>[2x]HHHHHHMKDRFELVSKYQPQGDQPKAIEKLVKGIQEGKKHQTLLGATGTGKTFTVSNLIKEVNKPTLVIAHNKTLAGQLYSEFKEFFPNNAVEYFVSYYDYYQPEAYVPQTDTFIEKDASINDEIDKLRHSATSALFERRDVIIIASVSCIYGLGSPEEYREMVVSLRTEMEIERNELLRKLVDIQYARNDIDFQRGTFRVRGDVVEIFPASRDEHCVRVEFFGDEIERIREVDALTGEILGDRDHVAIFPASHFVTRAEK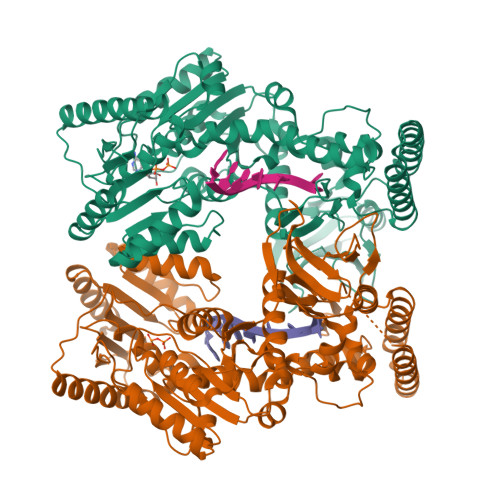MEKAIQNIEKELEEQLKVMHENGKLLEAQRLEQRTRYDLEMMREMGFCSGIENYSRHLTLRPPGSTPYTLLDYFPDDFMIVVDESHVTIPQVRGMFNGDQARKQVLVDHGFRLPSALDNRPLRFEEFEKHMHNIVYVSATPGPYEIEHTDEMVEQIIRPTGLLDPLIDVRPIEGQIDDLIGEIQARIERNERVLVTTLTKKMSEDLTDYLKEIGIKVNYLHSEIKTLERIEIIRDLRLGKYDVLVGINLLREGLDIPEVSLVAILDADKEGFLRSERSLIQTIGRAARNAEGRVIMYADKITKSMEIAINETKRRREQQERFNEEHGITPKTINKEIRDVIRATVAAEDKAEYKTKAAPKLSKMTKKERQKVVEQMEHEMKEAAKALDFERAAELRDLLLELKAEG> MSLRIGVIGT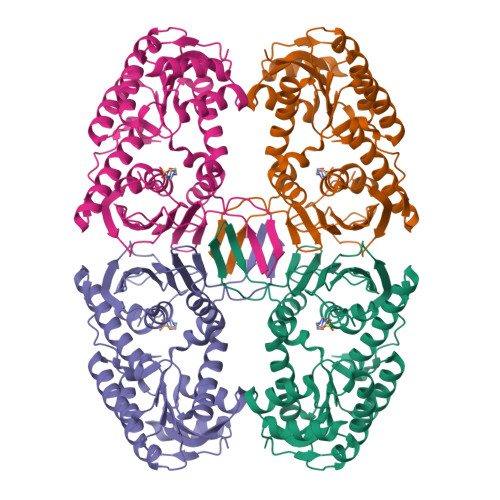GAIGKEHINRITNKLSGAEIVAVTDVNQEAAQKVVEQYQLNATVYPNDDSLLADENVDAVLVTSWGPAHESSVLKAIKAQKYVFCEVPLATTAEGCMRIVEEEIKVGKRLVQVGFMRRYDSGYVQLKEALDNHVIGEPLMIHCAHRNPTVGDNYTTDMAVVDTLVHEIDVLHWLVNDDYESVQVIYPKKSKNALPHLKDPQIVVIETKGGIVINAEIYVNCKYGYDIQCEIVGEDGIIKLPEPSSISLRKEGRFSTDILMDWQRRFVAAYDVEIQDFIDSIQKKGEVSGPTAWDGYIAAVTTDACVKAQESGQKEKVELKEKPEFYQSFTTVQN>[2x]MGSSHHHHHHSQDPDQVQYENTLKNFKIREQQFDNSWCAGFSMAALLNATKN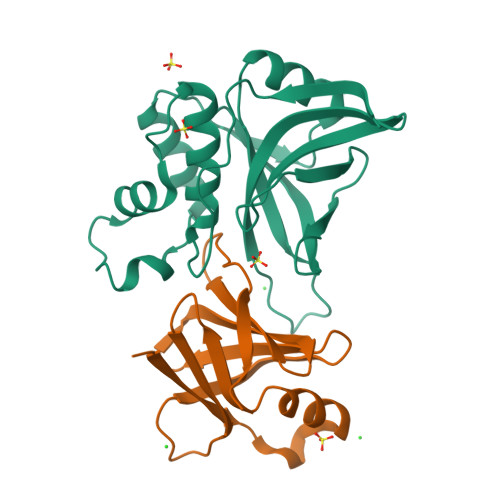TDTYNAHDIMRTLYPEVSEQDLPNCATFPNQMIEYGKSQGRDIHYQEGVPSYNQVDQLTKDNVGIMILAQSVSQNPNDPHLGHALAVVGNAKINDQEKLIYWNPWDTELSIQDADSSLLHLSFNRDYNWYGSMIGY;>MYQLQFINLVYDTTKLTHLEQTNINLFIGNWSNHQLQKSICIRHGDDTSHNQYHILFIDTAHQRIKFSSFDNEEIIYILDYDDTQHILMQTSSKQGIGTSRPIVYERLV[2x]> GMTILSDVKALGQQIWLDNLSRSLVQSGELAQMLKQGVCGVTSNPAIFQKAFAGDALYADEVAALKRQNLSPKQRYETMAVADVRAACDVCLAEHESTGGKTGFVSLEVSPELAKDAQGTVEEARRLHAAIARKNAMIKVPATDAGIDALETLVSDGISVNLTLLFSRAQTLKAYAAYARGIAKRLAAGQSVAHIQVVASFFISRVDSALDATLPDRLKGKTAIALAKAAYQDWEQYFTAPEFAALEAQGANRVQLLWASTGVKNPAYPDTLYVDSLIGVHTVNTVPDATLKAFIDHGTAKATLTESADEARARLAEIAALGIDVETLAARLQEDGLKQFEEAFEKLLAPLV

In the redox-sensitive enzyme transaldolase from Neisseria gonorrhoeae, the side chains of neighboring residues Lys 8 and Cys 38 at the protein surface form an NOS cross-link under oxidizing conditions that leads to a loss of enzymatic activity through ‘structural crosstalk’ with the active site. Under reducing conditions, the cross-link is disengaged, and enzymatic activity is restored. In the previously reported redox-sensitive transaldolase, the NOS bridge functions as an allosteric switch that changes the structure of the protein, including that of the active site, and thereby regulates enzymatic activity. We have recently reported the discovery of an allosteric lysine–cysteine redox switch with a covalent NOS bridge that regulates the enzymatic activity in response to changing redox conditions.

Next, we tested the impact of resolution and X-ray dose in X-ray crystallographic experiments on the traceability of covalent NOS bridges in protein structures. In the transaldolase protein crystals we analyzed, the NOS bridge exhibits almost full occupancy, and our system may therefore be regarded as a best-case scenario (also considering the low B-factors). To test the impact of high-energy synchrotron radiation on the NOS bridge in protein crystals, which is known to promote photochemical reactions of redox-sensitive groups, we conducted dose-dependent experiments depositing doses between 0.27 and 5.4 MGy in 0.27-MGy increments (X-ray crystallographic statistics in Supplementary Table 1). Photochemistry during data collection is unlikely to cause NOS bridge formation artificially; to the contrary, NOS bridges decompose while interacting with high-energy radiation but only at doses far higher than commonly used for data collection.> SDRVRSIT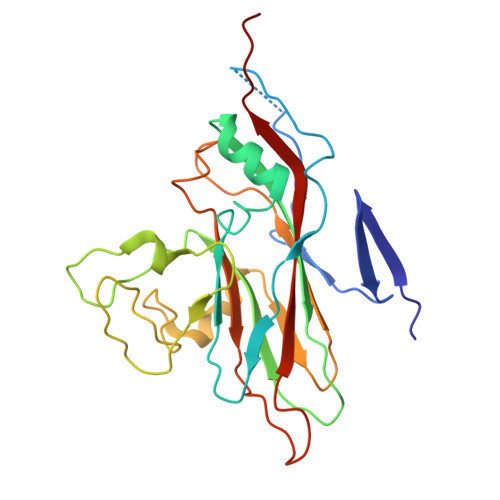LGNSTITTQESANVVVGYGVWPDYLSDEEATAEDQPTQPDVATCRFYTLDSVSWMKESQGWWWKFPDALRDMGLFGQNMQYHYLGRSGYTIHVQCNASKFHQGCLLVVCVPEAEMGAANINEKINREHLSNGEVANTFSGTKSSNTNDVQQAVFNAGMGVAVGNLTIFPHQWINLRTNNCATIVMPYINSVPMDNMFRHYNFTLMIIPFAKLDYAAGSSTYIPITVTVAPMCAEYNGLRLG Anopheles gambiae thioester-containing protein 1 (TEP1) is a complement-like protein that plays a central role in the opsonization of gram-negative bacteria in the hemolymph. TEP1 also binds to the surface of Plasmodium ookinetes that traverse the midgut epithelium following ingestion of an infectious blood meal, targeting those ookinetes for lysis and, in certain mosquito strains, melanization. TEP1 is composed of a series of eight macroglobulin (MG) domains, the β-sheet CUB domain and α-helical thioester domain (TED). The TED contains an intramolecular β-cysteinyl-γ-glutamyl thioester bond that is protected from inadvertent hydrolysis by sequestration within a protein-protein interface formed by the TED and MG8 domains.

Here we report the crystal structure of full-length TEP1*S1. The refined model of TEP1*S1 has three molecules, two of which (chains A, C) comprise residues 22–1338 with the exception of four gaps; residues 561–562, 575–582 in the linker (LNK) domain, 606–628 within the protease-sensitive region, and 822–829 in the CUB domain. A third molecule (chain B) with higher B-factors has poor or absent density for much of domains MG1, MG2, MG4, MG5 and MG6, but is otherwise complete for residues 629–1338 with the exception of 822–829 in the CUB domain. The overall structure of TEP1*S1 is very similar to that of TEP1*R1. The MG1, MG2, MG5 and MG6 domains also form a rigid body but are rotated 11° relative to TEP1*R1. The pre-α4 and catalytic loops form part of the TED-MG8 domain interface that protects the thioester from premature activation or hydrolysis. Both loops are ordered in the TEP1*S1 structure. The TEP1*R1 catalytic loop contains a sequence of five residues including Lys 966 and Glu 970 (966KAGAE970). These charged residues also occur in the TEP1*S1 catalytic loop but their positions are switched (966ETGKV970). TEP1*S1 Glu 966 adopts a different conformation than Lys 966 in TEP1*R1, directed into a pocket occupied by a Cl− ion in TEP1*R1, within hydrogen bonding distance of Ser 921 Oγ and Phe 923 N (the same conformation observed for Glu 1098 in complement factor C3). In the pre-α4 loop the substitution N919G permits a different backbone conformation for TEP1*S1 with Gly 919 O within hydrogen bonding distance of Val 914 N. The displacement of the catalytic loop in TEP1*S1 leads L914V to introduce a small cavity within the TED-MG8 interface between Trp 971 and the thioester bond.

>LLVVGPKFIRANQEYTLVISNFNSQLSKVDLLLKLEGETDNGLSVLNVTKMVDVRRNMNRMINFNMPEELTAGNYKITIDGQRGFSFHKEAELVYLSKSISGLIQVDKPVFKPGDTVNFRVILLDTELKPPARVKSVYVTIRDPQRNVIRKWSTAKLYAGVFESDLQIVPTPMLGVWNISVEVEGEELVSKTFEVKEYVLSTFDVQVMPSVIPLEEHQAVNLTIEANYHFGKPVQGVAKVELYLDDDKLNQKKELTVYGKGQVELRFDNFAMDADQQDVRVKVSFIEQYTNRTVVKQSQITVYRYAYRVELIKESPQFRPGLPFKCALQFTHHDGTPAKGITGKVEVSDVGFETTTTSDNDGLIKLELQPSEGTEQLGINFNAVDGFFFYEDVNKVETVTDAYIKLELKSPIKRNKLMRFMVTCTERMTFFVYYVMSKGNIIDAGFMRPNKQTKYLLQLNATEKMIPKAKILIATVAGRTVVYDYADLDFQELRNNFDLSIDEQEIKPGRQIELSMSGRPGAYVGLAAYDKALLLFNKNHDLFWEDIGQVFDGFHAINENEFDIFHSLGLFARTLDDILFDSANEKTGRNALQSGKPIGKLVSYRTNFQESWLWKNVSIGRSGSRKLIEVVPDTTTSWYLTGFSIDPVYGLGIIKKPIQFTTVQPFYIVENLPYSIKRGEAVVLQFTLFNNLGAEYIADVTLYNVANQTEFVGRPDTDLSYTKSVSVPPKVGVPISFLIKARKLGEMAVRVKASIMLGHETDALEKVIRVMPESLAQPKMDTSFFCFDDYKNQTFPFNLDINKKADNGSKKIEFRLNPNLLTMVIKNLDNLLAVPTGCGEQNMVKFVPNILVLDYLYATGSKEQHLIDKATNLLRQGYQNQMRYRQTDGSFGVWEKSGSSVFLTAFVATSMQTASKYMNDIDAAMVEKALDWLASKQHSSGRFDETGKVWHKDMQGGLRNGVALTSYVLTALLENDIAKVKHAVVIQNGMNYLSNQLAFINNPYDLSIATYAMMLNGHTMKKEALDKLIDMSISDNNKKERYWGTTNQIETTAYALLSFVMAEKYLDGIPVMNWLVNQRYVTGSFPRTQDTFVGLKALTKLAEKISPSRNDYTVQLKYKKNTKYFNINSEQIDVQNFLEIPEDTKKLEINVGGIGFGLLEVIYQFDLNLVNFEHRFKLDLEKQNTGSDYELRLRVCANYIPELTDSQSNMALIEVTLPSGYVVDRNPISEQTTVNPIQNMEIRYGGTSVVLYYYKMGTERNCFTVTAYRRFKVALKRPAYVVVYDYYNTNLNAIKVYEVDKQNVCEICEEEDCPAECHHHHHH[3x]> HHSGEHFEGEKVFRVNVEDENDISLLHELASTRQIDFWKPDSVTQIKPHSTVDFRVKAEDILAVEDFLEQNELQYEVLINNLRSVLEAQFDSRVRTTGHSYEKYNNWETIEAWTKQVTSENPDLISRTAIGTTFLGNNIYLLKVGKPGPNKPAIFMDCGFHAREWISHAFCQWFVREAVLTYGYESHMTEFLNKLDFYVLPVLNIDGYIYTWTKNRMWRKTRSTNAGTTCIGTDPNRNFDAGWCTTGASTDPCDETYCGSAAESEKETKALADFIRNNLSSIKAYLTIHSYSQMILYPYSYDYKLPENNAELNNLAKAAVKELATLYGTKYTYGPGATTIYPAAGGSDDWAYDQGIKY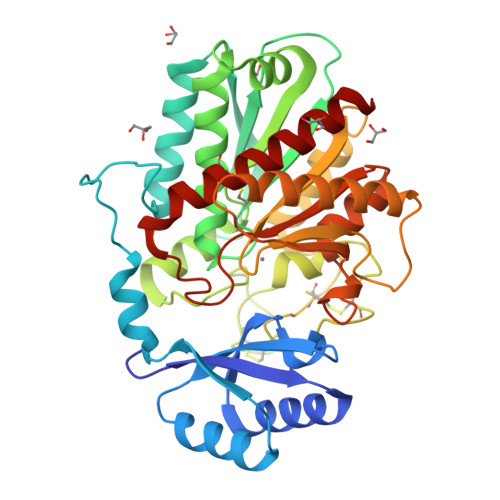SFTFELRDKGRYGFILPESQIQATCEETMLAIKYVTNYVLGHL> GSHMSDNPKVLVADDDKKIAQFIKTKFEENGIDTTVAFDGKEALFLINTNNYDVIVIDWMMPYLDGISLLKILRKQNINTPVIILSALDSTENKIEGLKSGSDDYLTKPFSIDELIIRVNILYKRTKQITEA

In summary, we conclude that Francisella BfpR is a response regulator of the OmpR/PhoP family that negatively regulates the expression of some FPI proteins and biofilm formation and positively regulates resistance to AMPs. Response regulators are transcription factors composed of two domains, a receiver (REC) domain which is connected to a DNA-binding domain through a flexible linker. On a molecular level, the response regulator propagates the signal by accepting the phosphate onto a conserved aspartate located within the REC domain. Alignments of FTN_452 to other bacterial response regulators suggest that FTN_1452 is a member of the OmpR/PhoP family.

The structure of the BfpR N-terminal REC domain (BfpRN) was solved using X-ray crystallography. The structure was refined to 1.80 Å resolution with a crystallographic Rwork of 0.1824 and Rfree of 0.2019. The BfpRN construct used for crystallization was composed of residues Met1 to Ala129 with three additional N-terminal residues remaining after cleavage of the affinity tag. Only residues Asn4 through Lys124 could be traced into the electron density. As expected from our sequence homology observations, the structure shares the canonical OmpR/PhoP receiver domain with an alternating α/β-fold consisting of 5-helices and 5-strands (Bourret, 2010). The asymmetric unit of BfpR contains one monomer with an adjacent symmetry mate forming the biologically relevant dimer. The dimer α4-β5-α5 interface of BfpR contains major salt bridges between Lys92 and Glu112, Asp102 and Arg116, and Asp101 and Arg123. The BfpR active site contains the canonical conserved aspartate residues, including the phosphorylation site at Asp55. A calcium ion is coordinated into the position of the active site magnesium. Alignment of active site residues of BfpR to BfmR bound to a phosphomimic results in an RMS of 0.290 Å.>[6x]SMEKTQETVQRILLEPYKYLLQLPGKQVRTKLSQAFNHWLKVPEDKLQIIIEVTEMLHNASLLIDDIEDNSKLRRGFPVAHSIYGIPSVINSANYVYFLGLEKVLTLDHPDAVKLFTRQLLELHQGQGLDIYWRD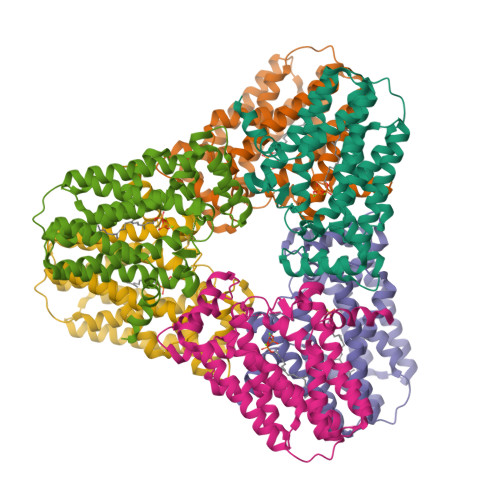NYTCPTEEEYKAMVLQKTGGLFGLAVGLMQLFSDYKEDLKPLLNTLGLFFQIRDDYANLHSKEYSENKSFCEDLTEGKFSFPTIHAIWSRPESTQVQNILRQRTENIDIKKYCVHYLEDVGSFEYTRNTLKELEAKAYKQIDARGGNPELVALVKHLSKMFKEENE Two Cas12i (Cas12i1 and Cas12i2) proteins have crRNA-guided dsDNA cleavage activity. In addition to the double-strand DNA (dsDNA) cleavage activity, Cas12i2 cleaves ssDNA in trans upon crRNA forming heteroduplex with the complementary ssDNA, as well as processes the pre-crRNA to form the mature crRNA. The Cas12i2 consists of the recognition (REC) and nuclease (NUC) lobes connected by the wedge (WED) domain. The RuvC domain is the sole DNase catalytic domain in Cas12i2, with catalytic residues Asp599, Glu833, and Asp1019 lining the active pocket.

In the DNA-bound Cas12i2 ternary complexes, a 5-nt ssDNA, which was probably introduced with the target DNA, is observed in the RuvC catalytic pocket. In addition, the ssDNA bound in the catalytic pocket remains intact may due to the high concentration of the complex and the chemicals used for crystallization, suggesting that our DNA-bound Cas12i2 complex is in the substrate binding state. The phosphate group between the 2nd and the 3rd nucleotides is located in the catalytic pocket, indicating that this is the cleavage position. In the Cas12i2wt–crRNA–DNA ternary complex, a pair of Mg2+ cations (A and B), separated by 4.0 Å, are located on either side of the scissile phosphate between nucleotides 2 and 3. Both metal ions coordinate the scissile phosphate group and RuvC domain catalytic residues. Mg2+A coordinates the side chains of Asp599, Asp1019, and Asn601, while Mg2+B coordinates with the side chains of Glu833 and Asp599. One water coordinating Mg2+A is positioned 3.9 Å away from the scissile phosphate, and is located approximately in line with the scissile phosphate and the leaving oxygen atom, suggesting this water acts as the nucleophile that attacks the phosphorus of the scissile phosphate. Mg2+B coordinates the 3′ oxygen atom leaving group, indicating the cleavage products contain 5′-phosphate and 3′-OH groups. Thus the two Mg ions facilitate DNA hydrolysis with Mg2+A coordinating and activating the water nucleophile, and Mg2+B stabilizes the leaving group. However, no metal ions were observed in these AacCas12b structures. Our Cas12i2wt–crRNA–DNA ternary complex with two metal ions bound in the RuvC catalytic pocket represents a substrate binding state of the catalytic pocket.

> SMSSAIKSYKSVLRPNERKNQLLKSTIQCLEDGSAFFFKMLQGLFGGITPEIVRFSTEQEKQQQDIALWCAVNWFRPVSQDSLTHTIASDNLVEKFEEYYGGTASDAIKQYFSASIGESYYWNDCRQQYYDLCRELGVEVSDLTHDLEILCREKCLAVATESNQNNSIISVLFGTGEKEDRSVKLRITKKILEAISNLKEIPKNVAPIQEIILNVAKATKETFRQVYAGNLGAPSTLEKFIAKDGQKEFDLKKLQTDLKKVIRGKSKERDWCCQEELRSYVEQNTIQYDLWAWGEMFNKAHTALKIKSTRNYNFAKQRLEQFKEIQSLNNLLVVKKLNDFFDSEFFSGEETYTICVHHLGGKDLSKLYKAWEDDPADPENAIVVLCDDLKNNFKKEPIRNILRYIFTIRQECSAQDILAAAKYNQQLDRYKSQKANPSVLGNQGFTWTNAVILPEKAQRNDRPNSLDLRIWLYLKLRHPDGRWKKHHIPFYDTRFFQEIYAAGNSPVDTCQFRTPRFGYHLPKLTDQTAIRVNKKHVKAAKTEARIRLAIQQGTLPVSNLKITEISATINSKGQVRIPVKFDVGRQKGTLQIGDRFCGYDQNQTASHAYSLWEVVKEGQYHKELGCFVRFISSGDIVSITENRGNQFDQLSYEGLAYPQYADWRKKASKFVSLWQITKKNKKKEIVTVEAKEKFDAICKYQPRLYKFNKEYAYLLRDIVRGKSLVELQQIRQEIFRFIEQDCGVTRLGSLSLSTLETVKAVKGIIYSYFSTALNASKNNPISDEQRKEFDPELFALLEKLELIRTRKKKQKVERIANSLIQTCLENNIKFIRGEGDLSTTNNATKKKANSRSMDWLARGVFNKIRQLAPMHNITLFGCGSLYTSHQDPLVHRNPDKAMKCRWAAIPVKDIGDWVLRKLSQNLRAKNIGTGEYYHQGVKEFLSHYELQDLEEELLKWRSDRKSNIPCWVLQNRLAEKLGNKEAVVYIPVRGGRIYFATHKVATGAVSIVFDQKQVWVCNADHVAAANIALTVKGIGEQSSDEENPDGSRIKLQLTS> MDMMMDKQEIKREYIEQEGHFETKSRRRELHIEILSEQTKSDIRNSKLVVMN;> PTHIAIG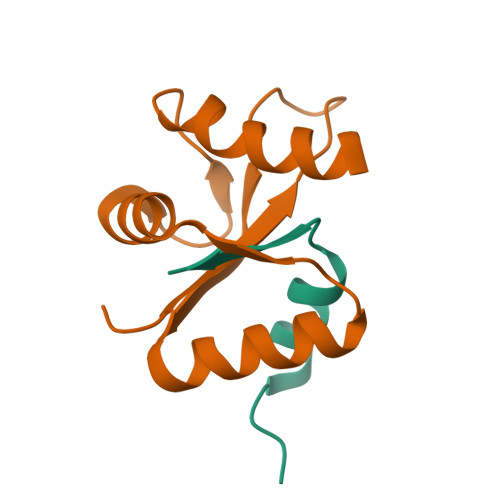IYFNPEIAPAPFISLIETNQCALAVRKYANEVGIPTVRDVKLARKLYKTHTKYSFVDFEHLDEVLRLIVWLEQVENTHLEHHHHHH>SASGVDDRDLLLAPKWISFLSLSSFLKQKLLSLLRQIRELRLTTTVYPPQDKLMWWSHCCDPEDIKVVILGQDPYHKGQATGLAFSVDPQCQVPPSLRSIFRELEASVPNFSTPSHGCLDSWARQGVLLLNTVLTVEKGRAGSHEGLGWDWFTSFIISSISSKLEHCVFLLWGRKAIDRTPLINAQKHLVLTAQHPSPLASLGGRHSRWPRFQ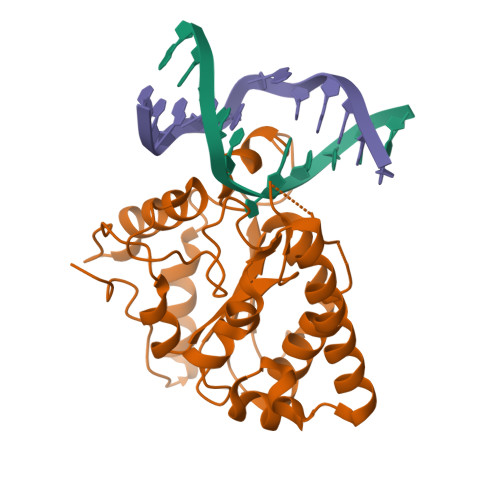GCNHFNLANDYLTRHRRETVDWGLLEQ[4x]> MGDRCAPIKASGVLIGDSVLVTDVEQARSLYSCGYYGQPLDVEKPRGADFEGPLRLSLIESLYLAEKGVLEVAKPDGSSVGVEDLRTAVRG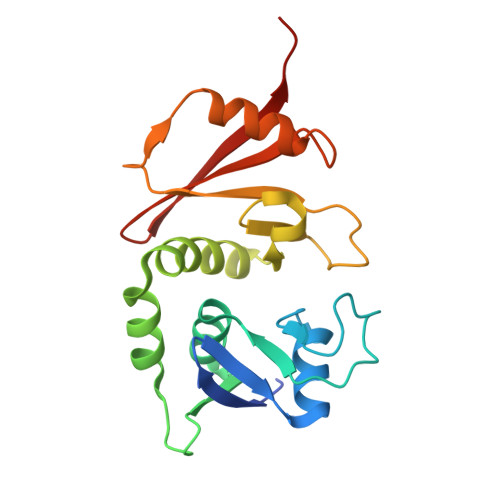NPRFSMLYNIYRDLRERGFVVRSGLKFGSDFAVYRLGPGIDHAPFIVHAYSPEDNIDPVEIVRAGRLSHSVRKKFVFAVTRGGDVSYLMIDWFRP LUMICHROME | C12 H10 N4 O2 | 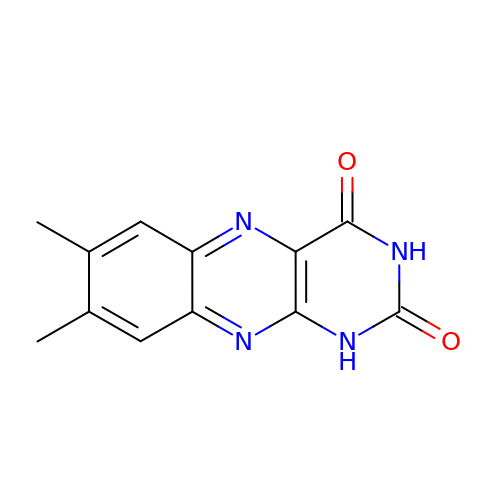ZJTJUVIJVLLGSP-UHFFFAOYSA-N>[3x]TSTKRFTCPEESEASNCSCEEFPSKTHFYCPDFNPTLYVDVEDRMRVDFKCYDEPHDFKSLPNLAIGSVKLLTVVDCVLDDDRPILESFKFLEVADVRSFVYNNHENGIRYNAKYFEGMEQLENLTLARGVVSIDRDTFSGFLNLKRLTIEHNKLNLQPGTFEALSNLTYLGLVYNGLNEIQPGLFDGLESLEALSLSYNDIKSLSAGSFNGLSSLRMLNLRVNKIESFDANTFASLKELSRLEITL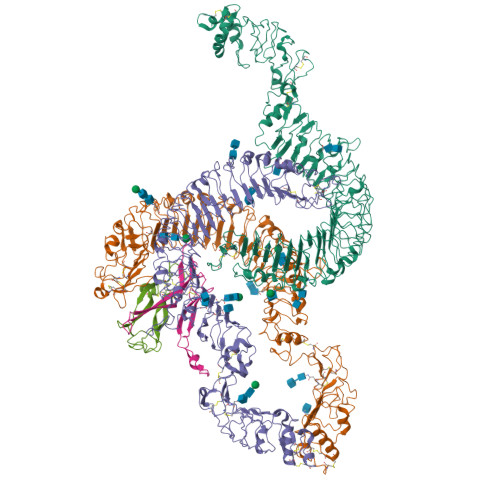NPFVSLPRGLFSENKKLKTLILTNNRKLVTLPEELLANLKELTVVNLSHNGVGNLPESLLSGSSGIIELNLGYNRLNSLPEELLSDQPQLQVLNLDHNQLESIPDYFLERNVELQTLYLSHNRLRSLSEKAFTKLKNLKELHLENNQLQTIPQFLFSGTPKLEEIYMQNNQLALHANSFINEELSIADNDNTPFQVLQKLRILHLRNNSISTIFQDWYINNLEMQSLDLSFNKLPGLSYTQLQFQSNITLNLSNNEISQVLLIDDLDLQPYQRINVDLNHNPLNCNCNALKFIQLIQSKAEHGLQFNVDQLRCSEPPNLLDATMDQLQTKDLLCDFESADDCPKDCQCAMRLLDHTVIVNCSGRGLTEFPDLPIPSQLHEDFNALEVHVENNRLTKLPNLTKHNEITQLYARNNSIQNLLPHNIPSKLRIIDLSQNLLKMIDDSTLAQINRSSHLETIRLSQNQWLCDCPASSFLIFVQQNSRLISDMSAIRCHPSGKSLDSITVNELCFEDYTTENLYFQ;>[2x]GSDTANAPFLCESEQLLIHPKEELSRNNSMVWIVNTKDYKQGVRIEKCLKRQLGKPCNFCDADTECKQLFHYRTLVAVDKVTKKPYKEQVLLPSCCKCAKILSTGWSHPQFEK> LVVHARASRYDRRKPPPPDLPSLLFDQRIVYLGMPLVPAVTELMVAELLYLEKQGATLPIEMLINSSGTTRQDGEILSFDSEGVALTSTMGFIKNPISTVNMGLAVGWSCVVLSFGRKGWRKSLPHSLAM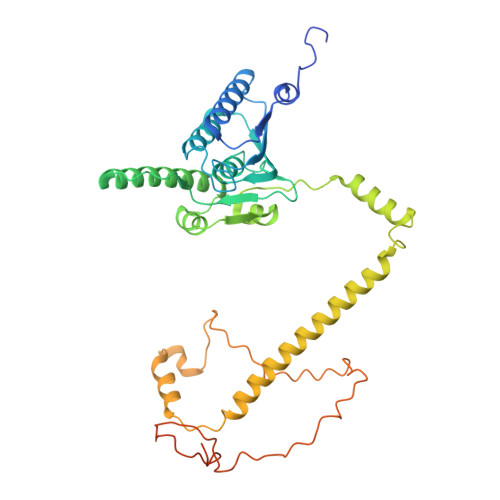IQQPRVPPTGQRQAIEVHIKWREVLDYKRELLRMFSLGTGLPVDKLDADMQRPLYMRPQDALEYGIIDEIIEPNEDKAEKAAQYWIRSGRAESEGRLEQWQEYLSLQEEYALKDSFRKVMTQDLRAAYRDTSSKLLKNSSRNMEQVQEFKERLPDDMLTENDEVRLPFSRDGVKLAILNAECYAERNIARQVAANKVSVPDKWRAAYAARPAPAAPAAEVDYDALIRAVEAMDEKAFATTDLDTLVEQYRVPA(2-MERCAPTOMETHYL-3-PHENYL-PROPIONYL)-GLYCINE | C12 H15 N O3 S | 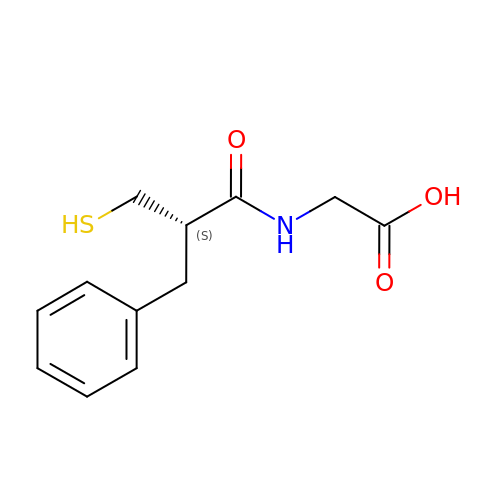LJJKNPQAGWVLDQ-SNVBAGLBSA-N> GSGAMAQNLDSMLHGTGMKSDSDQKKSENGVTLAPEDTLPFLKCYCSHHCPEDAINNTCITNGHCFTMIE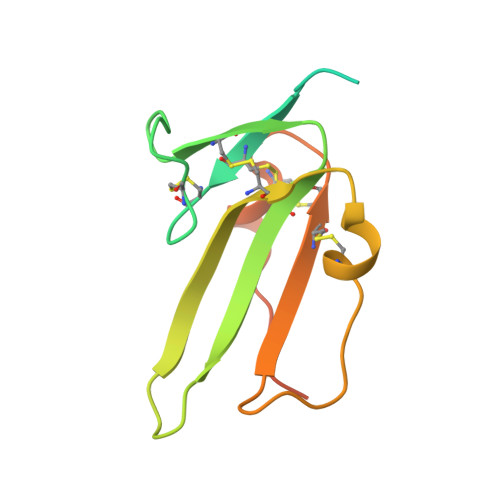EDDQGETTLTSGCLGLEGSDFQCRDTPIPHQRRSIECCRTNLCNQYLQPTLPPVVIGPFFDGSIR>[3x]MGHHHHHHMKSLRETESWKLLESSIIYYEGNPIGTVAAQDPELAALNYDQCFL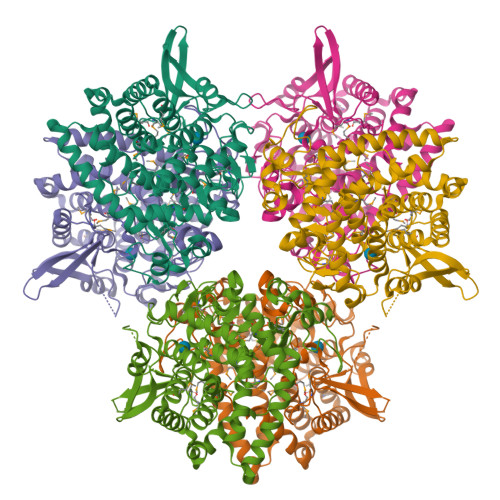RDFVPSAFVFLMDGQTDIVRNFLIETLTLQSHEKEMDCFQPGAGLMPASFKVESDGSKEYLVADFGEKAIARVPPVDSCMWWILLLRAYEKATGDLTLAREPKFQAGIKLILDLCLAHRFSMYPTMLVPDGAFMIDRRMGVYEHPLEIQVLFYAALRAARELLLPDGDGEQYLNKVHGRLGALQYHIRNYYWVDLKRLREIYRYKGNEFGKEIANKFNIFSQSIPDWVIEWLPEKGGYLAGNLGPGRMDFRFFALGNLMAILAGLASEEESQRIMNLFAHRWEDLIGYMPVKICYPALQGLEWQIVTGCDPKNIPWSYHNGGNWPVLLWLFTAAALKTGKVELAHEAIAIAEGRLSNDKFPEYYDGNNGRLIGKEARIYQTWSIAGLLVAKQFLANPDHVEFISFPDT>[2x]MKINDDIKELILEYMSRYFKFENDFYKLPGIKFTDANWQKFKNGGTDIEKMGAARVNAMLDCLFDDFELAMIGKAQTNYYNDNSLKMNMPFY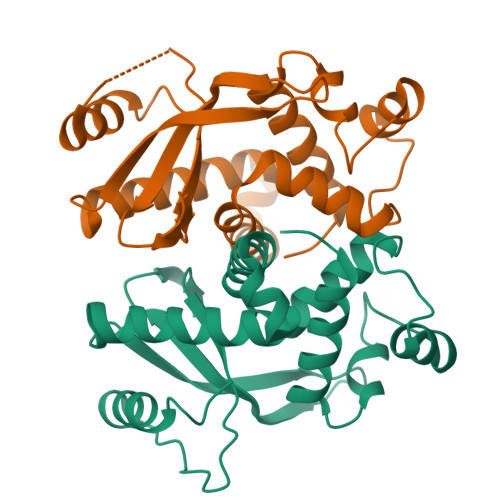TYYDMFKKQQLLKWLKNNRDDVIGGTGRMYTASGNYIANAYLEVALESSSLGSGSYMLQMRFKDYSKGQEPIPSGRQNRLEWIENNLENIRLE> ETGEEPPRFIKEPKDQIGVSGGVASFVCQATGDPKPRVTWNKKGKKVNSQRFETIEFDESAGAVLRIQPLRTPRDENVYECVAQNSVGEITVHAKLTVLREDQLPSGFPNIDMGPQLKVVERTRTATMLCAASGNPDPEITWFKDFLPVDPSASNGRIKQLRSGALQIESSEETDQGKYECVATNSAGVRYSSPANLYVRVRRVAPRFSILPMSHEIMPGGNVNITCVAVGSPMPYVKWMQGAEDLTPEDDMPVGRNVLELTDVKDSANYTCVAMSSLGVIEAVAQITVKSLPKAPGTPMVTENTATSITITWDSGNPDPVSYYVIEYKSKSQDGPYQIKEDITTTRYSIGGLSPNSEYEIWVSAVNSIGQGPPSESVVTRTGEQAPASAPRNVQARMLSATTMIVQWEEPVEPNGLIRGYRVYYTMEPEHPVGNWQKHNVDDSLLTTVGSLLEDETYTVRVLAFTSVGDGPLSDPIQVKTQ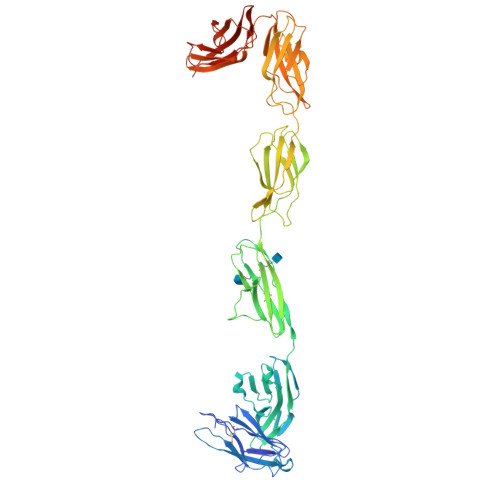QGVPGQPMNLRAEARSETSITLSWSPPRQESIIKYELLFREGDHGREVGRTFDPTTSYVVEDLKPNTEYAFRLAARSPQGLGAFTPVVRQRTLGTKHHHHHH> DPMKNTCKLLVVADHRFYRYMGRGEESTTTNYLIELIDRVDDIYRNTAWDNAGFKGYGIQIEQIRILKSPQEVKPGEKHYNMAKSYPNEEKDAWDVKMLLEQFSFDIAEEASKVCLAHLFTY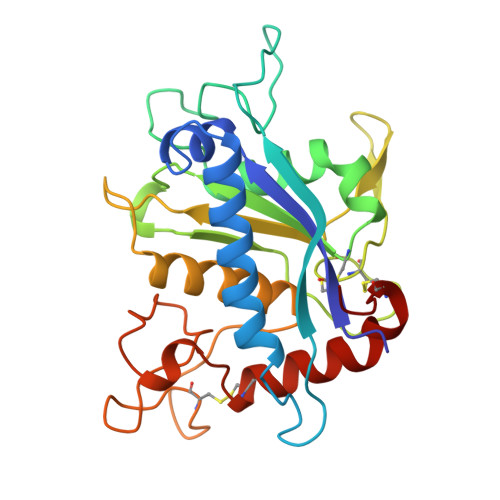QDFDMGTLGLAYVGSPRANSHGGVCPKAYYSPVGKKNIYLNSGLTSTKNYGKTILTKEADLVTTHELGHNFGAEHDPDGLAECAPNEEQGGKYVMYPIAVSGDHENNKMFSQCSKQSIYKTIESKAQECFQERS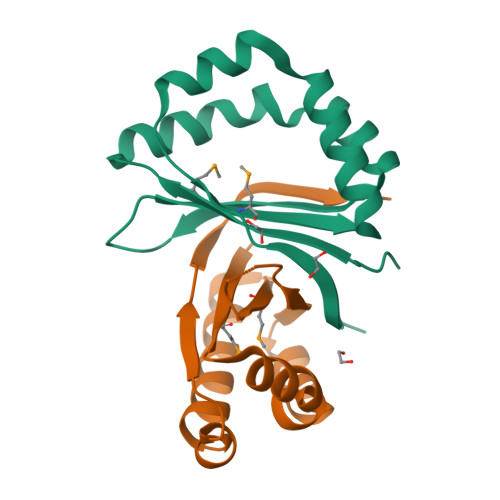>[6x]GMKDTDETAFLNSLFMDFTSENELELFLKSLDEVWSEDLYSRLSAAGLIRHVISKVWNKEQHRISMVFEYDSKEGYQKCQEIIDKEFGITLKEKLKKFVFKIHNNRGVVVSEFIRST>MHKSAFQALQGDIPTYEVNSSDEQDSDQDEEDVEQPSEPMHRLVSAPAASIHIEESKYISSNFSFDDDNTIYGHDYVIFGLKSNQNLIVKGQFVLEIQRGAIDINGVIYHSGVEPMKFINPSSSSIPLIQATQVLNSSLLENKESQENQHLFTPGYKSVIKLTNLDTHLESIGRVCPLFKNLFWQFDNFFAEDSLRLLDQYELAFSDYTFYPITKPDNTVSVIKHKNWMDVIKSLTELYSNDQSIKVIVIGGKNSGKSTFLRLLVQHMLSPTLQQLPINFMDLDPGQPEYSGTDCISLSKISEVQHGNHLSLTSTDSTQCHYVGFNSPKDQPTRYNLLVEQLVRSYESDGELKHESLLINTPGWIKGYGLELTRTLIERVKPTHVIYLNSGTLGVDIDIPKGTNLIPLQGSFNHSGSRYSSSQLRLLKTMAYFHKIDDFKFDFQPLLFSPPIQVSYGVSTGISALTHLKETGIGMDHLERSIEATIVGIFKVKRDHLEECELFNKGQLPLLPYKEFIKLSTEFFRLALVHSIDQEKKIMNLYIPQFRTLDLTKEAIIMVRGNTDLPIWEIASNEIVKRFKRQLPYITFEKGSSLEKKWKVRKNVQRRGQM[2x];>[2x]MNSHPRLTPWKSSDEVVYLKGLFFPADREQISRDELYRQYEEAISLVEMYSSRTRVSHILQSTAHLFSALMMLESFEGGLDDTVRLTASMTIIRFVNGLLDPNQQSQFAIPLHLLAKKIDLPSLFVEFRHSATHDALPSLEMCKTCVDRAIDWVWDHYWDGVLSIVEPQVETDDLEESLIKELKDLFKQYRRIRRQNITKLYKFGDSTPEGKEYWTCIAGIKDHADMANFYNVMIERIVSNKLKWEHLRALFEPMMNHFIHLKGWDFPLGLIDSMLSKNYEYSKFRGIDDTERAYLNDQEFKCAQKWIRWLAIEQIDRYDDVLVSKMIDTLGKTNHELNVEL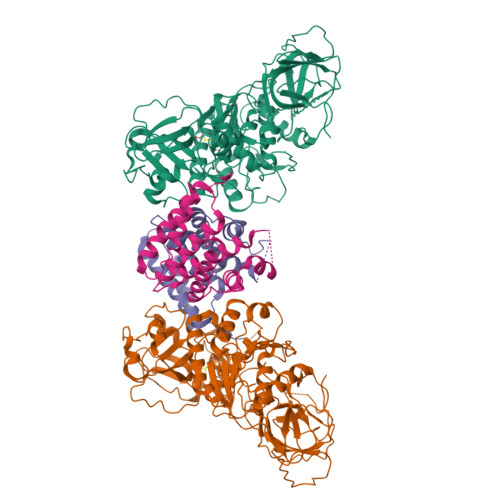LEKLQSRFSADPVIKDKIQAKLTLIQRLSTDTKTKRMNNLEDIMSDLESLKKRAKVTPTLHIKSFESHPNWTPKPFGVI>[6x]MQDRGNTVTIDFMSADGIVPGRTPVRYQGVEVGTVQDISLSDDLRKIEVKVSIKSDMKDALREETQFWLVTPKASLAGVSGLDALVGGNYIGMMPGKGKEQDHFVALDTQPKYRLDNGDLMIHLQAPDLGSLNSGSLVYFRKIPVGKVYDYAINPNKQGVVIDVLIERRFTDLVKKGSRFWNVSGVDANVSISGAKVKLESLAALVNGAIAFDSPEESKPAEAEDTFGLYEDLAHSQRGVIIKLELPSGAGLTADSTPLMYQGLEVGQLTKLDLNPGGKVTGEMTVDPSVVTLLRENTRIELRNPKLSLSDANLSALLTGKTFELVPG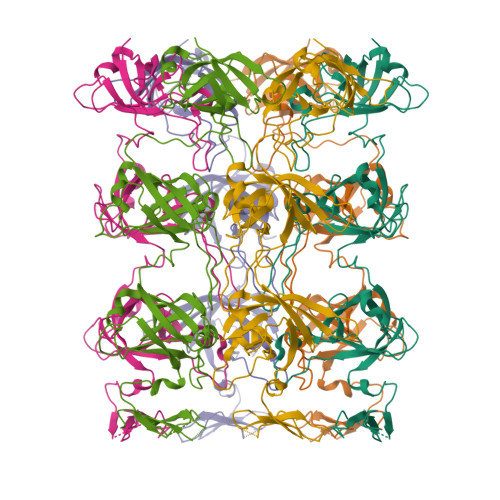DGEPRKEFVVVPGEKALLHEPDVLTLTLTAPESYGIDAGQPLILHGVQVGQVIDRKLTSKGVTFTVAIEPQHRELVKGDSKFVVNSRVDVKVGLDGVEFLGASASEWINGGIRILPGDKGEMKASYPLYANLEKALENSLSDLPTTTVSLSAETLPDVQAGSVVLYRKFEVGEVITVRPRANAFDIDLHIKPEYRNLLTSNSVFWAEGGAKVQLNGSGLTVQASPLSRALKGAISFDNLSGASASQRKGDKRILYASETAARAVGLSIIVEAPEAGSLGIGTPVLFRGLEVGTVTGMTLGTLSDRVMIAMRISKRYQHLVRNNSVFWLASGYSLDFGLTGGVVKTGTFNQFIRGGIAFATPPGTPLAPKAQEGKHFLLQESEPKEWREWGTALPKGETHHHHHH>GHMSNNFELKLQMSKVKGVSLHKFHLVNDLRGNLSVGEFEKDIPFTPKRYFTVFGVPNKEVRGEHAHKECKQFLICVSGNCSVLVDDGENREEYVLDSIDKGIYLPPMTWGVQYKYSKDAVL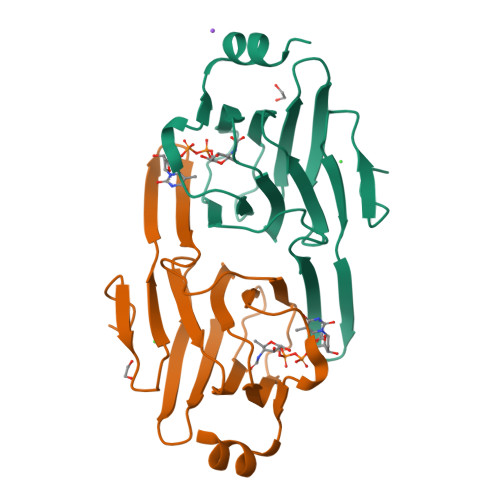LVFASHYYDSDDYIRDYSTFKQMRQN[6x]> MGSSHHHHHHLEVLFQGPVNALVSHLLVVEPEKLYAMPDPAGPDGHLPAVATLCDLFDREIVVTISWAKSIPGFSSLSLSDQMSVLQSVWMEVLVLGVAQRSLPLQDELA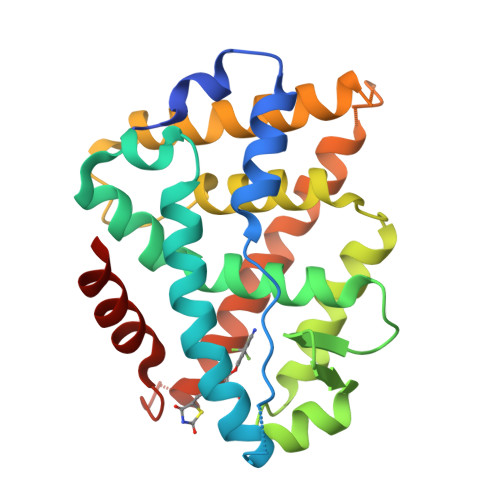FAEDLVLDEEGARAAGLGELGAALLQLVRRLQALRLEREEYVLLKALALANSDSVHIEDAEAVEQLREALHEALLEYEAGRAGPGGGAERRRAGRLLLTLPLLRQTAGKVLAHFYGVKLEGKVPMHKLFLEMLEAMMD> VVTYTTLIDGLAKAGRLEEALQLFQEMKEKGVKPDVVTYTTLIDGLAKAGRLEEALQLFQEMKEKGVKPDVVTYTTLIDGLAKAGRLEEALQLFQEMKEKGVKPDVVTYTTLIDGLAKAGRLEEALQLFQEMKEKGVKPDVVTYTTLIDGLAKAGRLEEALQLFEEMKEKGVKPDVVTYTTLIDG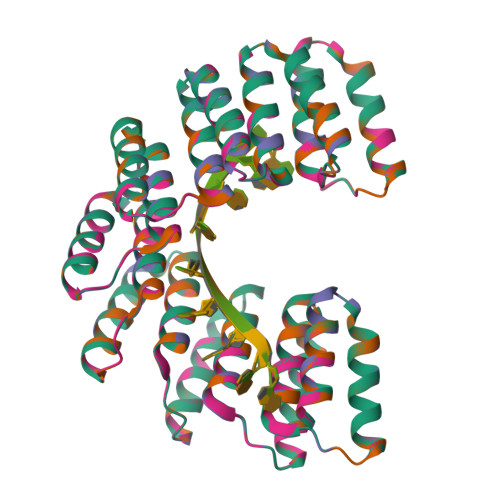LAKAGRLEEALQLFQEMKEKGVKPDVVTYTTLIDGLAKAGRLEEALQLFEEMKEKGVKPDVVTYTTLIDGLAKAGRLEEALQLFEEMKEKGVKPDVVTYTTLIDGLAKAGRLEEALQLFQEMKEKGVKPD;> VVTYNTLIDGLAKAGRLEEALQLFQEMKEKGVKPDVVTYNTLIDGLAKAGRLEEALQLFQEMKEKGVKPDVVTYNTLIDGLAKAGRLEEALQLFQEMKEKGVKPDVVTYNTLIDGLAKAGRLEEALQLFQEMKEKGVKPDVVTYNTLIDGLAKAGRLEEALQLFEEMKEKGVKPDVVTYNTLIDGLAKAGRLEEALQLFQEMKEKGVKPDVVTYNTLIDGLAKAGRLEEALQLFEEMKEKGVKPDVVTYNTLIDGLAKAGRLEEALQLFEEMKEKGVKPDVVTYNTLIDGLAKAGRLEEALQLFQEMKEKGVKPD;> VVTYTTLIDGLAKAGRLEEALQLFQEMKEKGVKPNVVTYTTLIDGLAKAGRLEEALQLFQEMKEKGVKPNVVTYTTLIDGLAKAGRLEEALQLFQEMKEKGVKPNVVTYTTLIDGLAKAGRLEEALQLFQEMKEKGVKPNVVTYTTLIDGLAKAGRLEEALQLFEEMKEKGVKPNVVTYTTLIDGLAKAGRLEEALQLFQEMKEKGVKPNVVTYTTLIDGLAKAGRLEEALQLFEEMKEKGVKPNVVTYTTLIDGLAKAGRLEEALQLFEEMKEKGVKPNVVTYTTLIDGLAKAGRLEEALQLFQEMKEKGVKPN;> VVTYNTLIDGLAKAGRLEEALQLFQEMKEKGVKPSVVTYNTLIDGLAKAGRLEEALQLFQEMKEKGVKPSVVTYNTLIDGLAKAGRLEEALQLFQEMKEKGVKPSVVTYNTLIDGLAKAGRLEEALQLFQEMKEKGVKPSVVTYNTLIDGLAKAGRLEEALQLFEEMKEKGVKPSVVTYNTLIDGLAKAGRLEEALQLFQEMKEKGVKPSVVTYNTLIDGLAKAGRLEEALQLFEEMKEKGVKPSVVTYNTLIDGLAKAGRLEEALQLFEEMKEKGVKPSVVTYNTLIDGLAKAGRLEEALQLFQEMKEKGVKPS>[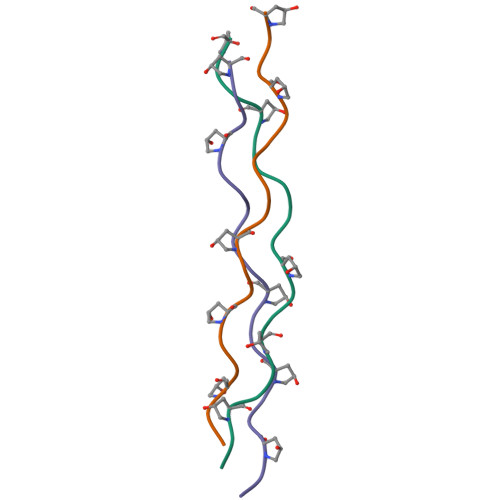3x]XGPPGPPGLPGEAGPPGPPX> GMDDLTNLAARLRLLEDREE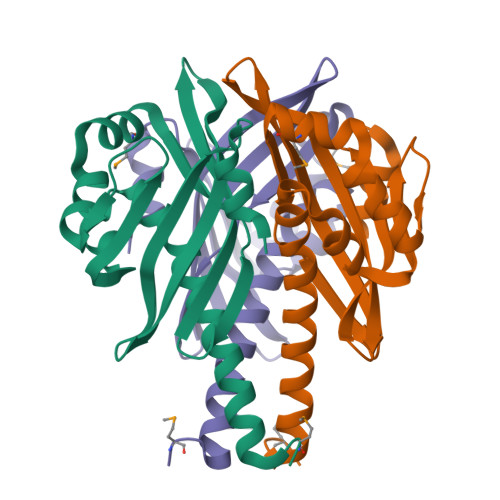IRELIARYGPLADSGDAEALSELWVEDGEYAVVGFATAKGRAAIAALIDGQTHRALMADGCAHFLGPATVTVEGDTATARCHSVVFRCVSGTFGSHRVSANRWTFRRTPAGWRAVRRENALLDGSAAARALLQFR> MKADNPFDLLLPAAMAKVAEEAGVYKATKHPLKTFYLAITAGVFISIAFVFYITATTGTGTMPFGMAKLVGGICFSLGLILCVVCGADLFTSTVLIVVAKASGRITWGQLAKNWLNVYFGNLVGALLFVLLMWLSGEYMTANGQWGLNVLQTADHKVHHTFIEAVCLGILANLMVCLAVWMSYSGRSLMDKAFIMVLPVAMFVASGFENSIANMFMIPMGIVIRDFASPEFWTAVGSAPENFSHLTVMNFITDNLIPVTIGNIIGGGLLVGLTYWVIYLRENDHH

FocA belongs to the widespread, evolutionarily ancient formate-nitrite transporter (FNT) family of pentameric anion channels and translocates formic acid bidirectionally. Central to the FNT family’s function are conserved histidine and threonine residues (H209 and T91 in E. coli FocA), both of which are essential for pH-dependent formate:H+ symport into fermenting E. coli cells. Here, we show the high-resolution structure of native E. coli FocA, together with the H209N variant, and describe the dynamic pore features that couple to the protonation state.

A FocA-H209N variant that exhibits an efflux-only channel-like function in vivo reveals a density consistent with formate located directly at N209, abolishing the channel’s amphiphilicity. The resolved structure of FocA-H209N at 2.97 Å (FSC = 0.143) exhibits minor structural differences compared with the native structure, but the polarity distribution across the pore is disturbed due to N209. The isolated FocA-H209N variant revealed the presence of a density close to N209, which would fit various small molecules, including formic acid. Capture of a potential translocation intermediate for FocA validates the disturbance of the polarity distribution across the pore, while in vivo experiments show that an E. coli strain with a mutation in codon 209 of the genomic copy of the focA gene, and which synthesizes FocA-H209N, has impaired growth due to reduced intracellular ATP levels, correlating with massive formic acid efflux. While the H209N FocA variant was found to be non-functional in vitro, in vivo experiments in the native environment demonstrate that it operates as an exceptionally efficient formic acid efflux channel, emphasizing the crucial role of H209 in pH-dependent formate uptake. Immunological analysis of plasmid-encoded FocA-H209N revealed that it is as stable as the native FocA protein15 and PflB is also stably produced in strain DH4200 (synthesizing FocA-H209N). These findings demonstrate that the amino acid exchange in FocA-H209N does not affect either synthesis or stability of the protein and has no indirect negative effect on FocA’s interaction partner, PflB. By placing the substrate at the additional density identified above, the results show preferential retention of formate close to the EM density due to the intrinsic property of formate being a hydrogen bond acceptor only. Cumulative analysis of all protomer channel contacts over all simulations performed showed that interactions around the EM density are highly prevalent. This indicates that this location is important for translocation, promoting the possibility that the captured density corresponds to the substrate.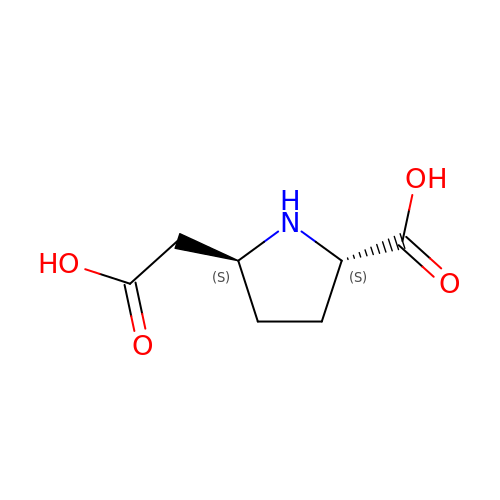(2S,5S)-5-CARBOXYMETHYLPROLINE | C7 H11 N O4 | LIZWYFXJOOUDNV-WHFBIAKZSA-N5-bromanyl-1,3-dihydroindol-2-one | C8 H6 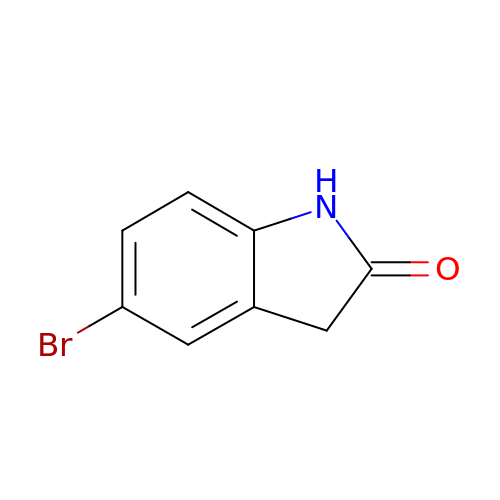Br N O | VIMNAEVMZXIKFL-UHFFFAOYSA-N>[2x]GPGSMSASRPNRVVLVLNSGSSSLKFQLVEPDSGMSRATGNIERIGEESSSVPDHDAALRRVFEILAEDDIDLQSCGLVAVGHRVVHGGKDFYEPTLLNDAVIGKLDELSPLAPLHNPPAVLCIRVARALLPDV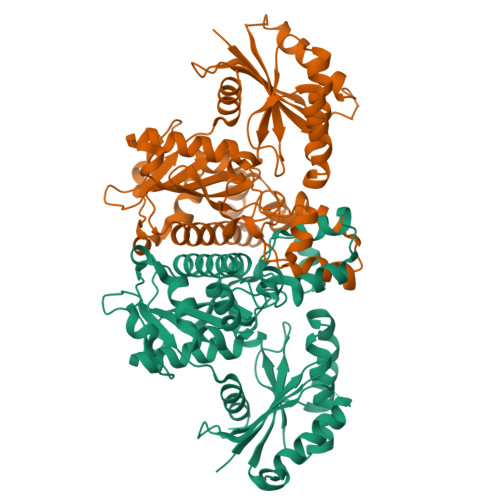PHIAVFDTAFFHQLPPAAATYAIDRELADVWKIRRYGFHGTSHEYVSQQAAEFLGKPIGDLNQIVLHLGNGASASAVAGGRPVETSMGLTPLEGLVMGTRSGDLDPGVIGYLWRTAKLGVDEIESMLNHRSGMLGLAGERDFRRLRAMIDDGDPAAELAYDVFIHRLRKYVGAYLAVLGHTDVVSFTAGIGEHDAAVRRDTLAGMAELGISLDERRNACPSGGARRISADDSPVTVLVIPTNEELAIARHCCSVLVA> MHHHHHHENLYF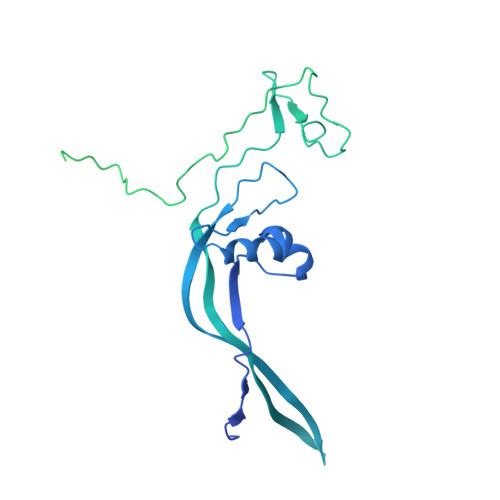QGMAAEAADLGLGAAVPVELRRERRMVCVEYPGVVRDVAKMLPTLGGEEGVSRIYADPTKRLELYFRPKDPYCHPVCANRFSTSSLLLRIRKRTRRQKGVLGTEAHSEVTFDMEILGIISTIYKFQGMSDFQYLAVHTEAGGKHTSMYDKVLMLRPEKEAFFHQELPLYIPPPIFSRLDAPVDYFYRPETQHREGYNNPPISGENLIGLSRARRPHNAIFVNFEDEEVPKQPLEAAAQTWRRVCTNPVDRKVEEELRKLFDIRPIWSRNAVKANISVHPDKLKVLLPFIAYYMITGPWRSLWIRFGYDPRKNPDAKIYQVLDFRIRCGMKHGYAPSDLPVKAKRSTYNYSLPITVKKTSSQLVTMHDLKQGLGPSGTSGARKPASSKYKLKDSVYIFREGALPPYRQMFYQLCDLNVEELQKIIHRNDGAENSCTERDGWCLPKTSDELRDTMSLMIRQTIRSKRPALFSSSAKADGGKEQLTYESGEDEEDEEEEEEEEEDFKPSDGSENEMETEILDYV> MKRRGEPLILVGEPSIKRNLLNEFDRIIENQEKSLKASKSTPDGTIKDRR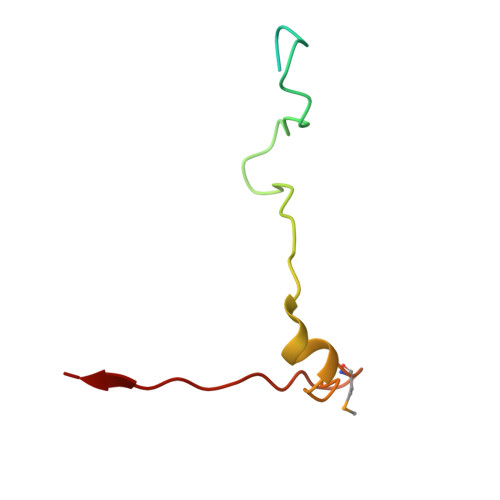LFMHHVSLEPITCVPF>[8x]MAVESRSRVTSKLVKAHRAMLNSVTQEDLKVDRLPGADYPNPSKKYSSRTEFRDKTDYIMYNPRPRDEPSSENPVSVSPLLCELAAARSRIHFNPTETTIGIVTCGGICPGLNDVIRSITLTGINVYNVKRVIGFRFGYWGLSKKGSQTAIELHRGRVTNIHHYGGTILGSSRGPQDPKEMVDTLERLGVNILFTVGGDGTQRGALVISQEAKRRGVDISVFGVPKTIDNDLSFSHRTFGFQTAVEKAVQAIRAAYAEAVSANYGVGVVKLMGRDSGFIAAQAAVASAQANICLVPENPISEQEVMSLLERRFCHSRSCVIIVAEGFGQDWGRGSGGYDASGNKKLIDIGVILTEKVKAFLKANKSRYPDSTVKYIDPSYMIRACPPSANDALFCATLATLAVHEAMAGATGCIIAMRHNNYILVPIKVATSVRRVLDLRGQLWRQVREITVDLGSDVRLARKLEIRRELEAINRNRDRLHEELAKL

Sequence comparisons of Trypanosoma spp. and Leishmania spp. show that divergence of the two genera involved amino acid substitutions that occur in the enzyme’s ‘reaching arms’ and ‘embracing arms’ that determine tetramer stability.

We also show that Leishmania PFK melts at a significantly lower (> 15 °C) temperature than Trypanosoma PFKs and that addition of either AMP or ATP results in a marked stabilization of the protein. The dramatic effects of AMP on Leishmania activity compared with the Trypanosoma PFKs may be explained by differences between the T‐to‐R equilibria for the two families, with the low‐melting Leishmania PFK favouring the flexible inactive T‐state in the absence of AMP. Sequence comparisons along with the enzymatic and structural data presented here also suggest there was a loss of AMP‐dependent regulation in Trypanosoma species rather than gain of this characteristic in Leishmania species and that AMP acts as a key regulator in Leishmania governing the balance between glycolysis and gluconeogenesis.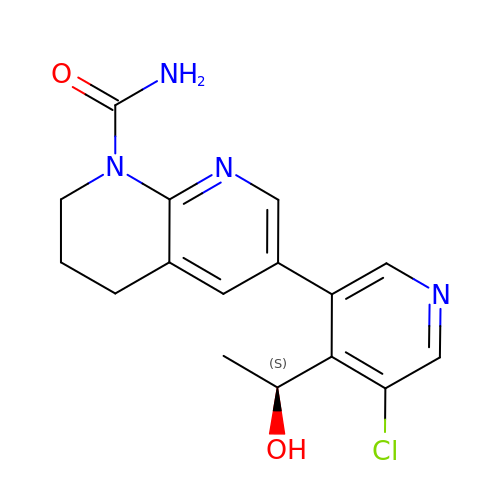6-[5-chloranyl-4-[(1~{S})-1-oxidanylethyl]pyridin-3-yl]-3,4-dihydro-2~{H}-1,8-naphthyridine-1-carboxamide | C16 H17 Cl N4 O2 | QDAISIXQQMBVSS-VIFPVBQESA-N The X-linked neuroligin 3 (NLGN3) gene encodes the postsynaptic adhesion molecule NLGN3, which interacts with presynaptic neurexins (NRXNs) to organize synaptogenesis. Here, we identified a non-canonical synapse-organizing interaction between NLGN3 and PTPδ splice variants lacking the meB peptide, which competed with NRXNs by steric hindrance. To elucidate the structural mechanism of the NLGN3–PTPδ-meB(–) interaction, we determined the crystal structures of mouse apo-NLGN3 ECD (residues 35–684) at 2.76 Å resolution and NLGN3 ECD in complex with PTPδA3B– Ig1–Fn1 at 3.85 Å resolution.

In the crystal of the NLGN3–PTPδA3B– complex, two adjacent NLGN3 molecules that are related by twofold crystallographic symmetry form a dimer in a manner similar to apo-NLGN3 ECD. Consequently, PTPδA3B– and NLGN3 form a W-shaped complex with a 2:2 stoichiometry. The Ig1–Ig3 domains of PTPδ interact extensively with the α/β-hydrolase-fold core of NLGN3. The NLGN3–PTPδ interface buries a surface of 1540 Å2 in total. In addition, the C-terminal tail of NLGN3 ECD lies on the meA3 insertion in PTPδ Ig2. The C-terminal tail of NLGN3 ECD is disordered in the apo-NLGN3 ECD structure, suggesting that it undergoes a disorder-to-order transition upon binding to PTPδ. The domain rearrangement of PTPδ Ig3 allows both PTPδ Ig2 and Ig3 to simultaneously interact with NLGN3. Our structural analyses suggest that the deletion of the meB peptide confines the spacing between Ig2 and Ig3 of PTPδ for simultaneous interaction with NLGN3, whereas the meA3 peptide in PTPδ Ig2 contributes to direct hydrophobic interaction with the C-terminal tail of the NLGN3 ECD. The binding site of NLGN3 for PTPδ Ig3 overlaps with the (potential) NRXN-binding site. The bound PTPδ Ig3 covers Gln370–Asp377.

> ETPPRFTRTPVDQTGVSGGVASFICQATGDPRPKIVWNKKGKKVSNQRFEVIEFDDGSGSVLRIQPLRTPRDEAIYECVASNNVGEISVSTRLTVLREDQIPRGFPTIDMGPQLKVVERTRTATMLCAASGNPDPEITWFKDFLPVDTSNNNGRIKQLRSESIGALQIEQSEESDQGKYECVATNSAGTRYSAPANLYVRVRRVPPRFSIPPTNHEIMPGGSVNITCVAVGSPMPYVKWMLGAEDLTPEDDMPIGRNVLELNDVRQSANYTCVAMSTLGVIEAIAQITVKALPKPPGTPVVTESTATSITLTWDSGNPEPVSYYIIQHKPKNSEEPYKEIDGIATTRYSVAGLSPYSDYEFRVVAVNNIGRGPASEPVLTQKHHHH;> PAPTVNTHFGKLRGARVPLPSEILGPVDQYLGVPYAAPPIGEKRFLPPEPPPSWSGIRNATHFPPVCPQNIHTAVPEVMLPVWFTANLDIVATYIQEPNEDCLYLNVYVPTEDGSGAKKQGEDLADNDGDEDEDIRDSGAKPVMVYIHGGSYMEGTGNMIDGSVLASYGNVIVITLNYRVGVLGFLSTGDQAAKGNYGLLDQIQALRWVSENIAFFGGDPRRITVFGSGIGASCVSLLTLSHHSEGLFQRAIIQSGSALSSWAVNYQPVKYTSLLADKVGCNVLDTVDMVDCLRQKSAKELVEQDIQPARYHVAFGPVIDGDVIPDDPEILMEQGEFLNYDIMLGVNQGEGLKFVEGVVDPEDGVSGTDFDYSVSNFVDNLYGYPEGKDTLRETIKFMYTDWADRDNPETRRKTLVALFTDHQWVEPSVVTADLHARYGSPTYFYAFYHHCQSLMKPAWSDAAHGDEVPYVFGVPMVGPTDLFPCNFSKNDVMLSAVVMTYWTNFAKTGDPNKPVPQDTKFIHTKANRFEEVAWSKYNPRDQLYLHIGLKPRVRDHYRATKVAFWKHLVPHLYNLHDMF> MRTHDDTWDIKTSVGTTAVMVAAARAAETDRPDALIRDPYAKLLVTNTG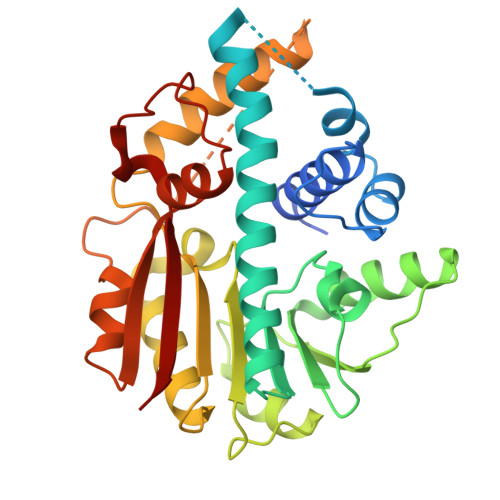AGALWEAMLDPSMVAKVEAIDAEAAAMVEHMRSYQAVRTNFFDTYFNNAVIDGIRQFVILASGLDSRAYRLDWPTGTTVYEIDQPKVLAYKSTTLAEHGVTPTADRREVPIDLRQDWPPALRSAGFDPSARTAWLAEGLLMYLPATAQDGLFTEIGGLSAVGSRIAVETSPLHGDEWREQMQLRFRRVSDALGFEQAVDVQELIYHDENRAVVADWLNRHGWRATAQSAPDEMRRVGRWGDGVPMADDKDAFAEFVTAHRL> GSHMRNVAAEQQLRELESTFDGRLGFVALDTATGARIAHRADERFPFCSTFKTMLSAAVLARSAGDAALLQRRIPYAKRDLVRYSPITEKHVGAGMTVAELCAATLQYSDNTAANLLIALLGGPQAVTAYARSIGDATFRLDRRETELNTAIPGDERDTTTPAAMAASVRRLPGDERDTTTPAAMAASVRRLLVGDALGTAQRAQLNAWMLGNKTGDARIRAGVPAGWRVADKTGTGDYGTGNDIGVAYPPDRAPIVFVVYTTMRSRNAQARDDVIASAARIAARAFV

In class A β-lactamases, a conserved structural element called the omega loop5 constitutes a wall at the active site that shapes the binding cavity. PenL (NCBI reference sequence: YP_439646.1) is highly conserved in pathogenic Burkholderia species, including Burkholderia pseudomallei, Burkholderia mallei, and Burkholderia cenocepacia. PenL has been used as a model in exploring various evolutionary paths to substrate spectrum extension through amino acid substitutions, deletions, and duplications. In this study, we demonstrate the extensive perturbation-absorbing capacity of the omega loop against TR mutations of various sizes, some of which are large enough to include the entire omega loop.

In contrast to the PenL-WT structure, in which every residue could be mapped, PenL-tTR10 and PenL-tTR11 both had a highly disordered region, where the mapping of the residues was not feasible due to high mobility. In PenL-tTR11, which has a longer tTR, nine residues in the upstream region of tTR11 were not mapped, in addition to the first repeat unit. In both PenL-tTR10 and PenL-tTR11, it appeared that the α10 helix structure (13 residues: 183–195) downstream of (in the case of PenL-tTR10) or overlapping (in the case of PenL-tTR11) the tTR required the second repeat unit of the tTR, instead of the first unit, to be in place in the protein backbone. In the PenL-tTR structures, perturbations in the omega loop resulted in the dislocation of a number of nearby residues, along with the disorganization of the α-helix in the omega loop (Glu166-Asn170), which most notably led to the breakage of a salt bridge that is normally present between Thr167 and Arg104 and tightly packs the active-site cavity. Asn170 was found to be further dislocated in PenL-tTR11, resulting in a wider opening in the active site cavity. Furthermore, the side chain of Asp240 was rotated approximately 90°, moving away from the active site by 3.21 Å in PenL-tTR10 and by 2.89 Å in PenL-tTR11. The precise volume of the active site in PenL-tTR11 could not be determined in the same manner because a key residue, Asn170, had swung away from the cavity. However, for the same reason, it is logical to assume that the active site in PenL-tTR11 is larger than that in PenL-tTR10. In contrast, the interaction between W1 and Glu166 was lost in PenL-tTR11. In this case, Lys73 may act as an alternative general base.> MATLTAKNLAKAYKGRRVVEDVSLTVNSGEIVGLLGPNGAGKTTTFYMVVGIVPRDAGNIIIDDDDISLLPLHARAR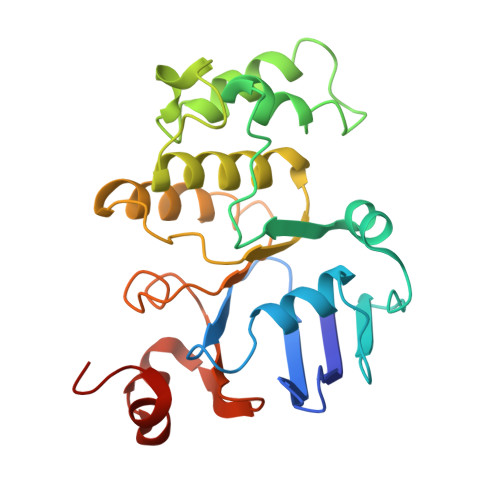RGIGYLPQEASIFRRLSVYDNLMAVLQIRDDLSAEQREDRANELMEEFHIEHLRDSMGQSLSGGERRRVEIARALAANPKFILLDEPFAGVDPISVIDIKRIIEHLRDSGLGVLITDHNVRETLAVCERAYIVSQGHLIAHGTPTEILQDEHVKRVYLGEDFRL> MMKMRWLSAAVMLTLYTSSSWAFSIDDVAKQAQSLAGKGYETPKSNLPSVFRDMKYADYQQIQFNHDKAYWNNLKTPFKLEFYHQGMYFDTPVKINEVTATAVKRIKYSPDYFTFGDVQHDKDTVKDLGFAGFKVLYPINSKDKNDEIVSMLGASYFRVIGAGQVYGLSARGLAIDTALPSGEEFPR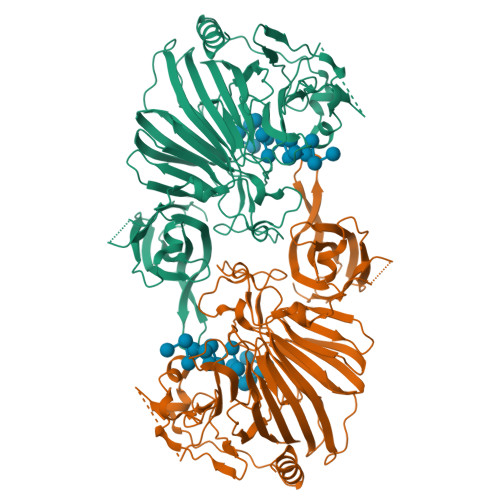FKEFWIERPKPTDKRLTIYALLDSPRATGAYKFVVMPGRDTVVDVQSKIYLRDKVGKLGVAPLTSMFLFGPNQPSPANNYRPELHDSNGLSIHAGNGEWIWRPLNNPKHLAVSSFSMENPQGFGLLQRGRDFSRFEDLDDRYDLRPSAWVTPKGEWGKGSVELVEIPTNDETNNNIVAYWTPDQLPEPGKEMNFKYTITFSRDEDKLHAPDNAWVQQTRRSTGDVKQSNLIRQPDGTIAFVVDFTGAEMKKLPEDTPVTAQTSIGDNGEIVESTVRYNPVTKGWRLVMRVKVKDAKKTTEMRAALVNADQTLSETWSYQLPANELEHHHHHH>MSELKTGHAGHNPWASVANSGPISILSYCGSSILMTVTNKFVVNLKDFNMNFVMLFVQSLVCTITLIILRILGYAKFRSLNKTDAKNWFPISFLLVLMIYTSSKALQYLAVPIYTIFKNLTIILIAYGEVLFFGGSVTSMELSSFLLMVLSSVVATW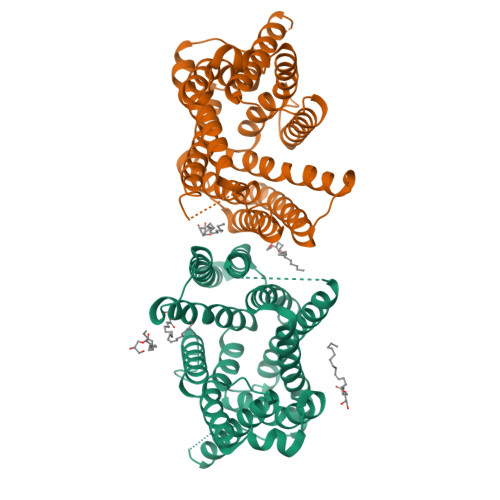GDQQAVAAKAASLAEGAAGAVASFNPGYFWMFTNCITSALFVLIMRKRIKLTNFKDFDTMFYNNVLALPILLLFSFCVEDWSSVNLTNNFSNDSLTAMIISGVASVGISYCSGWCVRVTSSTTYSMVGALNKLPIALSGLIFFDAPRNFLSILSIFIGFLSGIIYAVAKQKKQQAQPLRK[8x]> MEGAGQMAELPTHYGTIIKTLRKYMKLTQSKLSERTGFSQNTISN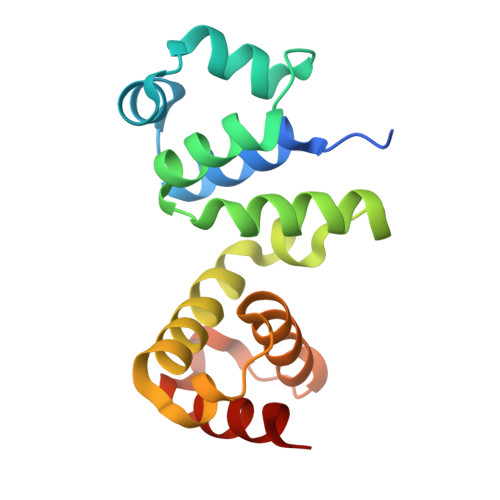HENGNRNIGVNEIEIYGKGLGIPSYILHRISDEFKEKGYSPTLNDFGKFDKMYSYVNKAYYNDGDIYYSSYDLYDETIKLLELLKESKINVNDIDYDYVLKLYKQILSTDT> WNNIVFYSLGDVN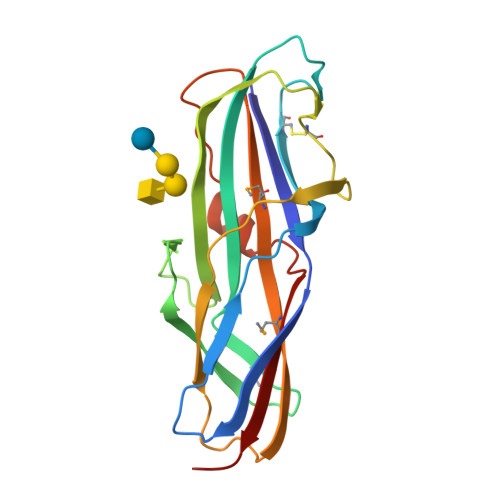SYQGGNVVITQRPQFITSWRPGIATVTWNQCNGPEFADGFWAYYREYIAWVVFPKKVMTQNGYPLFIEVHNKGSWSEENTGDNDSYFFLKGYKWDERAFDAGNLCQKPGEITRLTEKFDDIIFKVALPADLPLGDYSVKIPYTSGMQRHFASYLGARFKIPYNVAKTLPRENEMLFLFKNIGG> GSDYIIKEKTVLLQKKDSEGFGFVLRGAKAQTPIEEFTPTPAFPALQYLES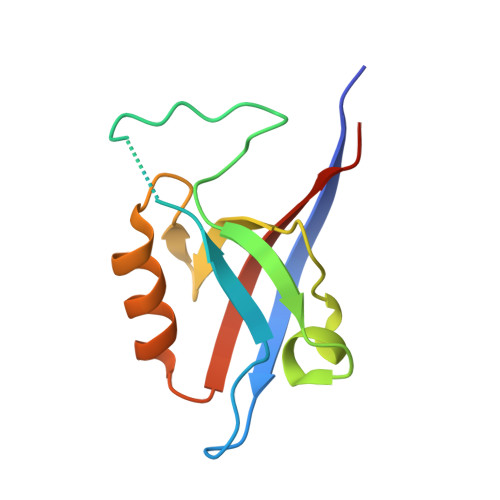VDEGGVAWRAGLRMGDFLIEVNGQNVVKVGHRQVVNMIRQGGNTLMVKVVMVTRHPDM> MPTKAVTFYEDINYGGASVSLQPGNYTLSQLNTAKIPNDWMTSLKVPSGWTVDVYENDNFTGTKWTYTSDTPWV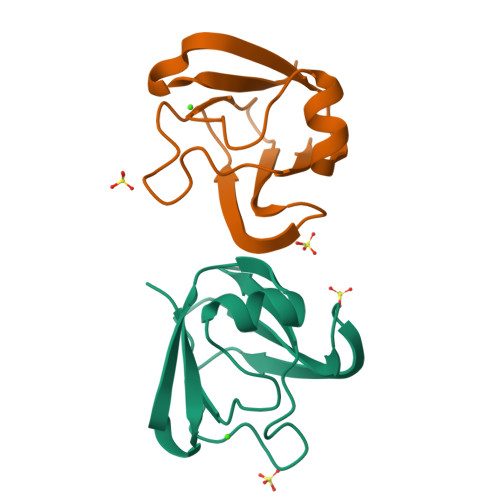GNDANDKMRSVKIYSTTNTGGDT> GPGSMAQTLINDTFLRALLREPTDYTPIWLMRQAGRYLPEYNATRARAGSFLGLAKHPDYATEVTLQPLERFPLDAAILFSDILTIPDAMGLGLDFAAGEGPKFAHPVRTEADVAKLAVPDIGATLGYVTDAVREIRRALTDGEGRQRVPLIGFSGSPWTLACYMVEGGGSDDFRTVKSMAYARPDLMHRILDVNAQAVAAYLNAQIEAGAQAVMIFDTWGGALADGAYQRFSLDYIRRVVAQLKR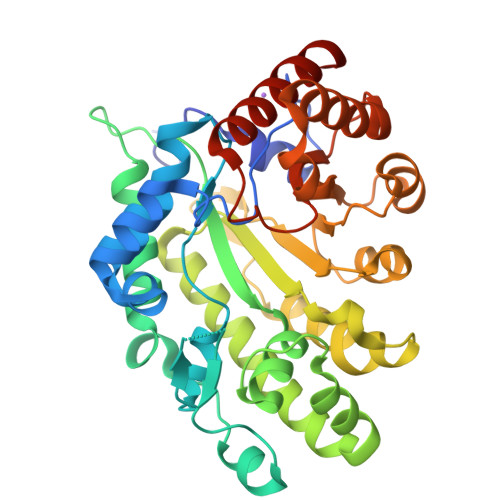EHDGARVPAIAFTKGGGLWLEDLAATGVDAVGLDWTVNLGRARERVAGRVALQGNLDPTILFAPPEAIRAEARAVLDSYGNHPGHVFNLGHGISQFTPPEHVAELVDEVHRHSRAIRSGTGS> XA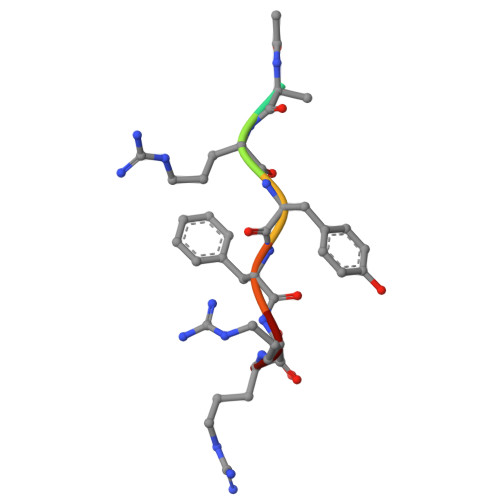RYFRR We previously showed that TacT is a Gcn5 N-acetyltransferase (GNAT) toxin that controls Salmonella growth through acetylation of aminoacyl-tRNA molecules. TacT acetylates the primary amine group of the amino acid on charged tRNA molecules, thereby blocking peptide bond formation and protein synthesis. A third-related toxin, TacT3, showing 28.3% of the amino acid identity to TacT, is conserved across serovars. We show that all three toxins induce the persister state by inhibiting translation through acetylation of aminoacyl-tRNAs.

We obtained the crystal structure of purified TacT3Y143F in 1.5 Å resolution. The fold of TacT3 appeared to be that of an acetyltransferase similar to TacT. with the exception of an additional C-terminal alpha-helix. Similarly to our results with TacT, purified TacT3 forms a dimer with a comparable dimerization interface. Examination of the surface electrostatic potential of TacT2 and TacT3 revealed a positively charged groove, leading from the active site of one monomer to another patch of positive charge on the second molecule of the dimer —features also present at the surface of TacT. Accordingly, for each toxin, a single amino acid substitution of the predicted catalytic site responsible for transfer of the acetyl moiety to the acceptor molecule (Y137F for TacT2SEn and Y143F for TacT3) completely abolished the toxicity in Salmonella. Single amino acid substitution of R88G and R94E in TacT2SEn and TacT3, respectively, abolished the toxicity in Salmonella, in agreement with our previous data for TacT. TacT3 appeared to be the most potent toxin, and comparison of its active site with that of TacT revealed a difference in the orientation of Ac-CoA. The adenine moiety is bent and more engaged in the binding pocket of TacT (and the modelled TacT2) compared to that of TacT3, most likely owing to the bulky side chain of the Trp142 residue present in TacT3. In TacT3, the adenine base of Ac-CoA is further stabilized outside the binding pocket by a hydrogen bond between its amine group and a carbonyl oxygen of the Gly145 residue. It is possible that this different conformation allows rapid unloading of coenzyme A after transfer of the acetyl moiety to the target substrate, increasing the processivity of the enzyme.

>GSMFTDWHEAAIGKTHNRMNFDCGDADLNQFLQRHARQNHEKGTTKTYVALDNSDVTRIHGFYSVSPASLIYAQVPGAISKGLGRYDVPVFRLGRLAVDKSMQGQGLGAQLLLSAGKRCIQAALQVGGVALLIDAKNKQVCDWFKGFGAVPLNDQPLSLLLSFKTLYAALSASGRL[2x]>M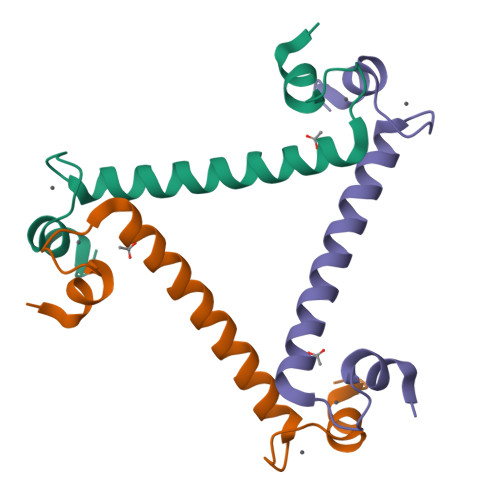AEALFKEIDVNGDGAVSYEEVKAFVSKKRAIKNEQLLQLIFKSIDADGNGEIDQNEFAKFYGSIQGQDLSDDKIGLKVLYKLMDVDGDGKLTKEEVTSFFKKHGIEKVAEQVMKADANGDGYITLEEFLEFSL[2x]Here, we investigate the capability of a deep neural network model to automate design of sequences onto protein backbones, having learned directly from crystal structure data and without any human-specified priors. To assess whether the model could perform sequence design for de novo structures, we tested our method on a Rosetta-generated four-fold symmetric de novo TIM-barrel backbone, a (βαβα)4 topology consisting of an eight-stranded barrel surrounded by eight alpha helices. We had the model fully redesign 50 four-fold symmetric sequences for the backbone and selected 8 designs for further characterization based on ranking by the model PLL and other metrics (see “Methods” section), using no information about previously confirmed sequences. Of these 8 designs, 4 are cooperatively folded proteins, as indicated by circular dichroism (CD) wavelength scans and by the presence of clear two-state transitions in thermal melt curves.

In the structure, we see that the C-terminal His tag for F2C interacts with the surface of the beta-barrel, which might also contribute to the dislodging of the C-terminal helix, although 3 of the 4 symmetric subunits are folded as expected. To elucidate this, we crystallized the protein with an N-terminal His-TEV tag (F2N, 1.58 Å resolution). Since the structure is a closed toroid, the N- and C-termini are proximal, and we see that the N-terminal tag is partially resolved folded against the barrel, displacing the C-terminal helix.

> HHHHHHENLYFQSDIAIVDADNPADAIQQVKDLRKYGAKLIAYKSKSSEELKLALKAGADIAIVDADNPADAIQQVKDLRKYGAKLIAYKSKSSEELKLALKAGADIAIVDADNPADAIQQVKDLRKYGAKLIAYKSKSSEELKLALKAGADIAIVDADNPADAIQQVKDLRKYGAKLIAYKSKSSEELKLALKAG2-(3-fluoro-4-methyl-anilino)-4-methyl-quinolin-5-ol | C17 H15 F N2 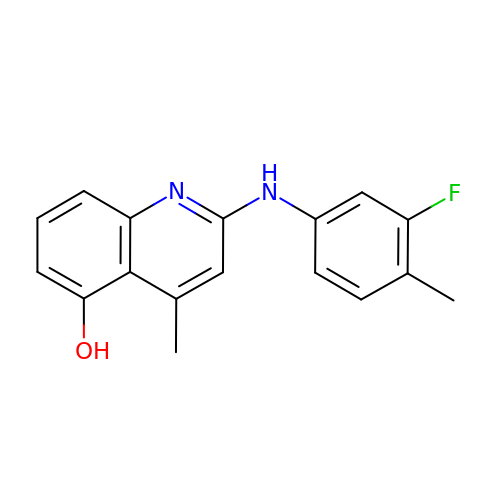O | YIACXICIQWGRMA-UHFFFAOYSA-N>SLDNSRTRPRVGHIQFLNCLPLYWGLARTGTLLDFELTKDTPEKLSEQLVRGDLDIGPVTLVEFLKNADDLVAFPDIAVG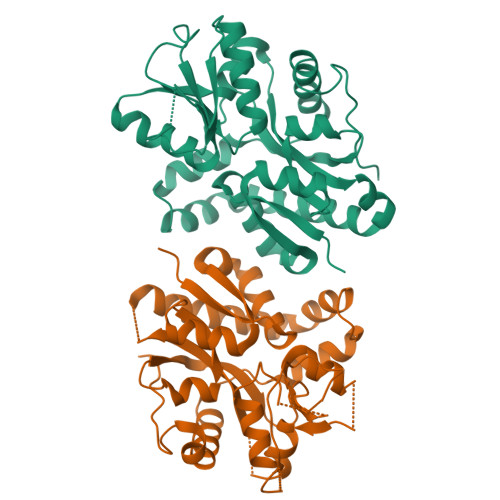CDGPVMSCVIVSQVPLDRLDGARVALGSTSRTSVRLAQLLLSERFGVQPDYYTCPPDLSLMMQEADAAVLIGDAALRANMIDGPRYGLDVHDLGALWKEWTGLPFVFAVWAARRDYAEREPVITRKVHEAFLASRNLSLEEVEKVAEQAARWEAFDEDTLAKYFTTLDFRFGAPQLEAVTEFARRVGPTTGFPADVKVELLKPEGHHHHHH[4x]>MKPEVEQELAHILLTELLAYQFASPVRWIETQDVFLKDFNTERVVEIGPSPTLAGMAQRTLKNKYESYDAALSLHREILCYSKDAKEIYYTPDPSELAAKEEPAKEEAPAPTPAASAPAPAAAAPAPVAAAAPAAAAAEIADEPVKASLLLHVLVAHKLKKSLDSIPMSKTIKDLVGGKSTVQNEILGDLGKEFGTTPEKPEETPLEELAETFQDTFSGALGKQSSSLLSRLISSKMPGGFTITVARKYLQTRWGLPSGRQDGVLLVALSNEPAARLGSEADAKAFLDSMAQKYASIVGVDLSSAASASGAAGAGAAAGAAMIDAGALEEITKDHKVLARQQLQVLARYLKMDLDNGERKFLKEKDTVAELQAQLDYLNAELGEFFVNGVATSFSRKKARTFDSSWNWAKQSLLSLYFEIIHGVLKNVDREVVSEAINIMNRSNDALIKFMEYHISNTDETKGENYQLVKTLGEQLIENCKQVLDVDPVYKDVAKPTGPKTAIDKNGNITYSEEPREKVRKLSQYVQEMALGGPITKESQPTIEEDLTRVYKAISAQADKQDISSSTRVEFEKLYSDLMKFLESSKEIDPSQTTQLAGMDVEDALDKDSTKEVASLPNKSTISKTVSSTIPRETIPFLHLRKKTPAGDWKYDRQLSSLFLDGLEKAAFNGVTFKDKYVLITGAGKGSIGAEVLQGLLQGGAKVVVTTSRFSKQVTDYYQSIYAKYGAKGSTLIVVPFNQGSKQDVEALIEFIYDTEKNGGLGWDLDAIIPFAAIPEQGIELEHIDSKSEFAHRIMLTNILRMMGCVKKQKSARGIETRPAQVILPMSPNHGTFGGDGMYSESKLSLETLFNRWHSESWANQLTVCGAIIGWTRGTGLMSANNIIAEGIEKMGVRTFSQKEMAFNLLGLLTPEVVELCQKSPVMADLNGGLQFVPELKEFTAKLRKELVETSEVRKAVSIETALEHKVVNGNSADAAYAQVEIQPRANIQLDFPELKPYKQVKQIAPAELEGLLDLERVIVVTGFAEVGPWGSARTRWEMEAFGEFSLEGCVEMAWIMGFISYHNGNLKGRPYTGWVDSKTKEPVDDKDVKAKYETSILEHSGIRLIEPELFNGYNPEKKEMIQEVIVEEDLEPFEASKETAEQFKHQHGDKVDIFEIPETGEYSVKLLKGATLYIPKALRFDRLVAGQIPTGWNAKTYGISDDIISQVDPITLFVLVSVVEAFIASGITDPYEMYKYVHVSEVGNCSGSGMGGVSALRGMFKDRFKDEPVQNDILQESFINTMSAWVNMLLISSSGPIKTPVGACATSVESVDIGVETILSGKARICIVGGYDDFQEEGSFEFGNMKATSNTLEEFEHGRTPAEMSRPATTTRNGFMEAQGAGIQIIMQADLALKMGVPIYGIVAMAATATDKIGRSVPAPGKGILTTAREHHSSVKYASPNLNMKYRKRQLVTREAQIKDWVENELEALKLEAEEIPSEDQNEFLLERTREIHNEAESQLRAAQQQWGNDFYKRDPRIAPLRGALATYGLTIDDLGVASFHGTSTKANDKNESATINEMMKHLGRSEGNPVIGVFQKFLTGHPKGAAGAWMMNGALQILNSGIIPGNRNADNVDKILEQFEYVLYPSKTLKTDGVRAVSITSFGFGQKGGQAIVVHPDYLYGAITEDRYNEYVAKVSAREKSAYKFFHNGMIYNKLFVSKEHAPYTDELEEDVYLDPLARVSKDKKSGSLTFNSKNIQSKDSYINANTIETAKMIENMTKEKVSNGGVGVDVELITSINVENDTFIERNFTPQEIEYCSAQPSVQSSFAGTWSAKEAVFKSLGVKSLGGGAALKDIEIVRVNKNAPAVELHGNAKKAAEEAGVTDVKVSISHDDLQAVAVAVSTKK[3x];>MDAYSTRPLTLSHGSLEHVLLVPTASFFIASQLQEQFNKILPEPTEGFAADDEPTTPAELVGKFLGYVSSLVEPSKVGQFDQVLNLCLTEFENCYLEGNDIHALAAKLLQENDTTLVKTKELIKNYITARIMAKRPFDKKSNSALFRAVGEGNAQLVAIFGGQGNTDDYFEELRDLYQTYHVLVGDLIKFSAETLSELIRTTLDAEKVFTQGLNILEWLENPSNTPDKDYLLSIPISCPLIGVIQLAHYVVTAKLLGFTPGELRSYLKGATGHSQGLVTAVAIAETDSWESFFVSVRKAITVLFFIGVRCYEAYPNTSLPPSILEDSLENNEGVPSPMLSISNLTQEQVQDYVNKTNSHLPAGKQVEISLVNGAKNLVVSGPPQSLYGLNLTLRKAKAPSGLDQSRIPFSERKLKFSNRFLPVASPFHSHLLVPASDLINKDLVKNNVSFNAKDIQIPVYDTFDGSDLRVLSGSISERIVDCIIRLPVKWETTTQFKATHILDFGPGGASGLGVLTHRNKDGTGVRVIVAGTLDINPDDDYGFKQEIFDVTSNGLKKNPNWLEEYHPKLIKNKSGKIFVETKFSKLIGRPPLLVPGMTPCTVSPDFVAATTNAGYTIELAGGGYFSAAGMTAAIDSVVSQIEKGSTFGINLIYVNPFMLQWGIPLIKELRSKGYPIQFLTIGAGVPSLEVASEYIETLGLKYLGLKPGSIDAISQVINIAKAHPNFPIALQWTGGRGGGHHSFEDAHTPMLQMYSKIRRHPNIMLIFGSGFGSADDTYPYLTGEWSTKFDYPPMPFDGFLFGSRVMIAKEVKTSPDAKKCIAACTGVPDDKWEQTYKKPTGGIVTVRSEMGEPIHKIATRGVMLWKEFDETIFNLPKNKLVPTLEAKRDYIISRLNADFQKPWFATVNGQARDLATMTYEEVAKRLVELMFIRSTNSWFDVTWRTFTGDFLRRVEERFTKSKTLSLIQSYSLLDKPDEAIEKVFNAYPAAREQFLNAQDIDHFLSMCQNPMQKPVPFVPVLDRRFEIFFKKDSLWQSEHLEAVVDQDVQRTC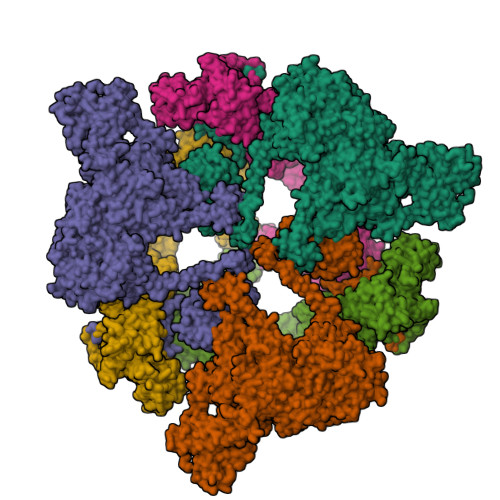ILHGPVAAQFTKVIDEPIKSIMDGIHDGHIKKLLHQYYGDDESKIPAVEYFGGESPVDVQSQVDSSSVSEDSAVFKATSSTDEESWFKALAGSEINWRHASFLCSFITQDKMFVSNPIRKVFKPSQGMVVEISNGNTSSKTVVTLSEPVQGELKPTVILKLLKENIIQMEMIENRTMDGKPVSLPLLYNFNPDNGFAPISEVMEDRNQRIKEMYWKLWIDEPFNLDFDPRDVIKGKDFEITAKEVYDFTHAVGNNCEDFVSRPDRTMLAPMDFAIVVGWRAIIKAIFPNTVDGDLLKLVHLSNGYKMIPGAKPLQVGDVVSTTAVIESVVNQPTGKIVDVVGTLSRNGKPVMEVTSSFFYRGNYTDFENTFQKTVEPVYQMHIKTSKDIAVLRSKEWFQLDDEDFDLLNKTLTFETETEVTFKNANIFSSVKCFGPIKVELPTKETVEIGIVDYEAGASHGNPVVDFLKRNGSTLEQKVNLENPIPIAVLDSYTPSTNEPYARVSGDLNPIHVSRHFASYANLPGTITHGMFSSASVRALIENWAADSVSSRVRGYTCQFVDMVLPNTALKTSIQHVGMINGRKLIKFETRNEDDVVVLTGEAEIEQPVTTFVFTGQGSQEQGMGMDLYKTSKAAQDVWNRADNHFKDTYGFSILDIVINNPVNLTIHFGGEKGKRIRENYSAMIFETIVDGKLKTEKIFKEINEHSTSYTFRSEKGLLSATQFTQPALTLMEKAAFEDLKSKGLIPADATFAGHSLGEYAALASLADVMSIESLVEVVFYRGMTMQVAVPRDELGRSNYGMIAINPGRVAASFSQEALQYVVERVGKRTGWLVEIVNYNVENQQYVAAGDLRALDTVTNVLNFIKLQKIDIIELQKSLSLEEVEGHLFEIIDEASKKSAVKPRPLKLERGFACIPLVGISVPFHSTYLMNGVKPFKSFLKKNIIKENVKVARLAGKYIPNLTAKPFQVTKEYFQDVYDLTGSEPIKEIIDNWEKYEQS[3x]>[4x]AVKYYTLEEIQKHNNSKSTWLILHYKVYDLTKFLEEHPGGEEVLREQAGG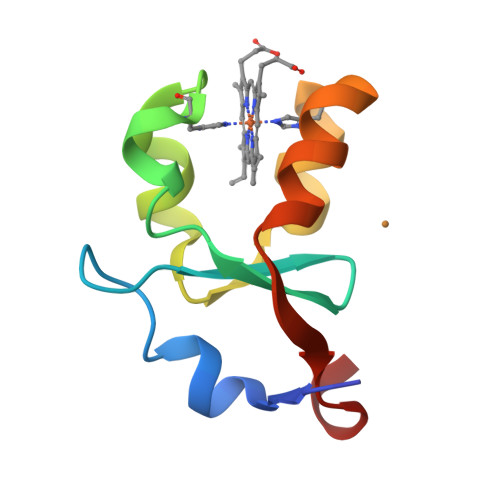DATENFEDVGHSTDARELLKTFIIGELHPDDR> GHMLRHIQNSLGSVYRSNTATPQGQIIHHRNFQSQFDTTGNTLYNNAWVCSLNVIKSRDGNNYSALEDITSDNQAFNNILEGIDIIECENLLKEMNVQKIPESSLFTNIKEALQAEVFNSTVEDDFESFISYELQNHGPLMLIRPSLGSECLHAECIVGYDSEVKKVLIYDSMNTSPEWQSNIDVYDKLTLAFNDKYKNEDCSICGLYYDGVYEPKPLHSSSWKDWCTIL;> METREHLFKVLVIGELGVGKTSIIKRYVHQLFSQHYRATIGVDFALKVLNWDSRTLVRLQLWDIAGQERFGNMTRVYYKEAVGAFVVFDISRSSTFEAVLKWKSDLDSKVHLPNGSPIPAVLLANKCDQNKDSSQSPSQVDQFCKEHGFAGWFETSAKDNINIEEAARFLVEKILVNHQSFPN

The protein GtgE has been identified as a cysteine protease that targets members of the Rab-family. Rab32 is involved in controlling the biogenesis of lysosome-related organelles (LRO). It is believed that GtgE inactivates Rab32 proteolytically and thereby prevents the delivery of antimicrobial factors that would impair Salmonella infection. Furthermore, by using a combination of biochemical characterization, molecular dynamics simulation, and binding studies, we demonstrate that GtgE shows exclusive selectivity for the inactive GDP-bound state of Rab32.

The high affinity of GtgEC45A for Rab32:GDP allowed us to purify thecomplex. Crystals obtained after reductively alkylating the truncated Rab3218-201:GDP:GtgE21-214,C45A-complex and the full-length complex Rab321-225:GDP:GtgE1-228,C45A diffracted up to 2.3 Å and 2.9 Å resolution, respectively. The X-ray structures of the complexes were solved by the molecular replacement technique using the coordinates of Rab32:GppCH2p (PDB ID: 4CYM17) and truncated GtgE (PDB ID: 4MI77) as appropriate search models (see Supplementary Table 1 for data collection and refinement statistics). The average B-factor of the full-length complex is higher than for the truncated complex, though the entire electron density is well defined for both structures.>[2x]GSFEL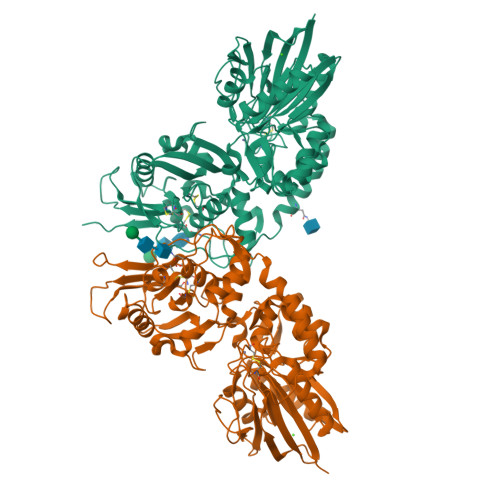TILHTNDVHARLEQTSRDSGKCTGEDCYGGVARRATKIRQIRASHRNVLLLDAGDQYQGTIWFNYYKGREVVHFMNSLRYDAMALGNHEFDNGLNGLLDPLLKNVKFPILSANIRPKGPIASNISGYILPYKIINVGSEKVGIIGYTTKETPVLSNPGPYLEFRDEVEELQKHADKLTTLGVNKIIALGHSGFMEDCRIAQKVKGVDVVVGGHTNTFLYTGSPPSNEVAAGNYPFMQLSDDGRQVPVVQAYAFGKYLGYLNVTFDDKGKVIKASGNPILLNKSIQEDPAVKAEISRMKVQLQNYSSQEIGRTIVYLNGTTHACRFHECNLGNLICDAVVYNNLRHPDDNEWNHVSMCIVNGGGIRSPIDEQANNGIITLEELTAVLPFGGTFDLLQIKGSTLRQAFEHSVHRHGQGTGELLQVSGIKVVYDLSQKPGKRVVSLNVLCTECRVPTYVPLEMEKTYKVLLPSFLAAGGDGYYMLKGDSSNHSSGDLDISIVGDYIKRMGKVFPAMEGRMVFSAGSL(~{N}~{E})-2-acetamido-~{N}-prop-2-enylidene-ethanamide | C7 H10 N2 O2 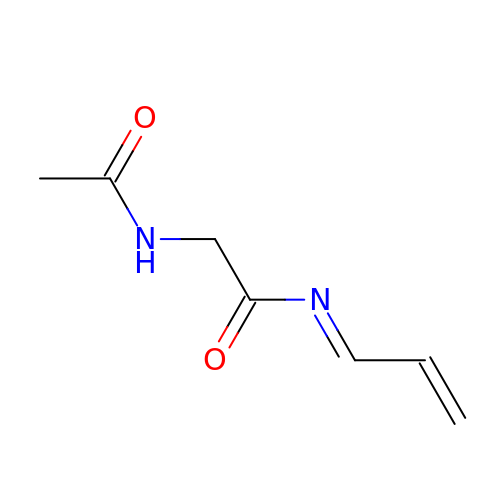| DSHANFFIVIVYBG-XBXARRHUSA-N> GPGYQDPKGRLYGTIGIQKRFYVSIDKIPEHVIN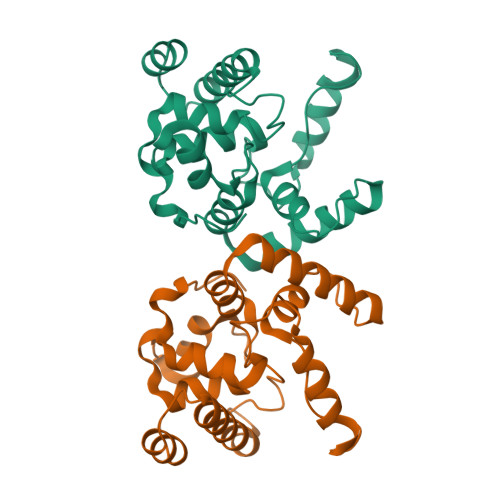AFVATEDRNFWHHFGIDPVAIVRAAIVNYRAGRIAQGGSTITQQLAKNLFLTRERTLERKIKEALLAIKIERTFDKKKIMELYLNQIYLGSGAYGVEAAAQVYFGKHVWELSLDEAALLAALPKAPAKYNPFYHPERALQRRNLVLKRMLEEGYITPEQYEEAVNK>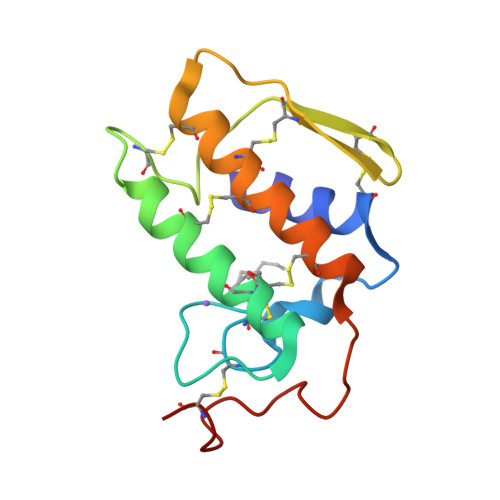 NLYQLMNMIQCANTRTWPSYTNYGCYCGKGGSGTPVDDLDRCCYTHDHCYNDAKNIDGCNPVTKTYSYTCTEPTITCNDSKDKCARFVCDCDRTAAICFAKAPYNTSNVMIRSTNSCQ>[2x]APQQINDIVHRTITPLIEQQKIPGMAVAVIYQGKPYYFTWGYADIAKKQPVTQQTLFELGSVSKTFIGVLGG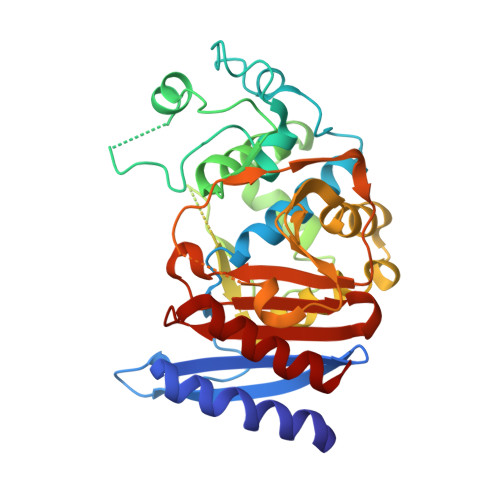DAIARGEIKLSDPTTKYWPELTAKQWNGITLLHLATYTAGGLPLQVPDEVKSSSDLLRFYQNWQPAWAPGTQRLYANSSIGLFGALAVKPSGLSFEQAMQTRVFQPLKLNHTWINVPPAEEKNYAWGYREGKAVHVSPGALDAEAYGVKSTIEDMARWVQSNLKPLDINEKTLQQGIQLAQSRYWQTGDMYQGLGWEMLDWPVNPDSIINGSDNKIALAARPVKAITPPTPAVRASWVHKTGATGGFGSYVAFIPEKELGIVMLANKNYPNPARVDAAWQILNALQ> SRIISRIAQELRRXGDE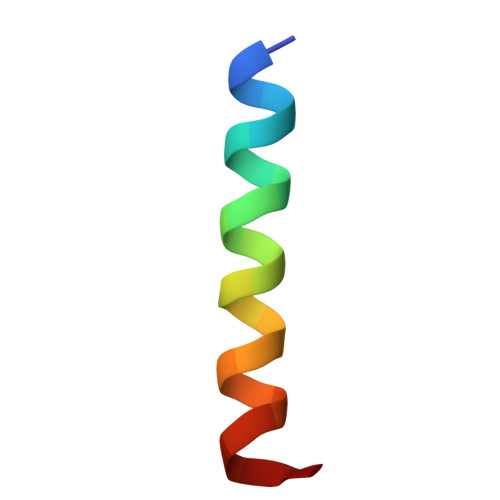FNATYA> GPLGSMAVTITLKTLQQQTFKIRMEPDETVKVLKEKIEAEKGRDAFPVAGQKLIYAGKILSDDVPIRDYRIDEKNFVVVMV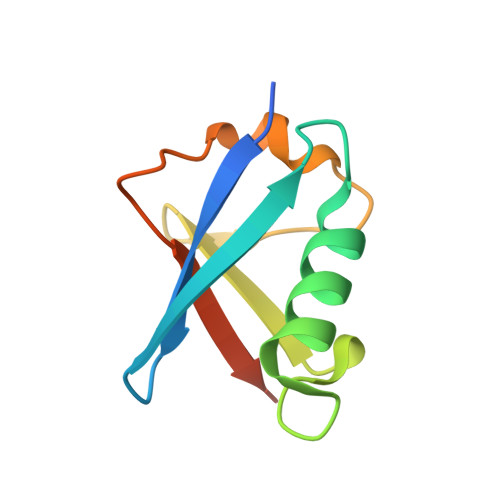TKTKAGQG~{N}8-(2,2-dimethylpropyl)-~{N}2-[2-ethoxy-4-(4-methyl-1,2,4-triazol-3-yl)phenyl]-6-methyl-pyrido[3,4-d]pyrimidine-2,8-diamine 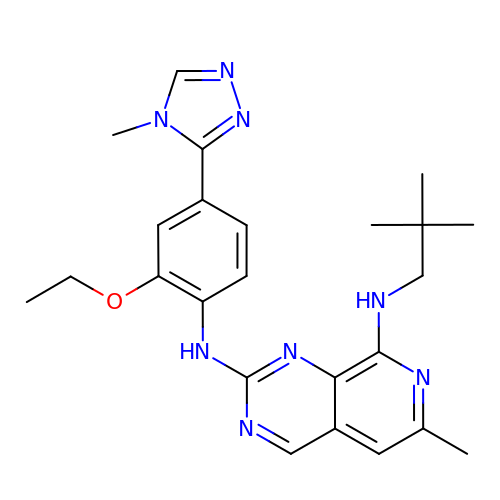| C24 H30 N8 O | SGWLRDAOCLITOM-UHFFFAOYSA-N> NVAYPLGEGLLSFAESLESQKIHFTTEVITSRIEPANRYVAEKLRITPGQDILYLERLRSIGDEKAMLIENRINIELCPGIVEIDFNQHNLFPTIESLSKRKIRYSESRYAARLIGNERGHFLDISEDAPVLHLEQLVFFSRELPVEFGNVWL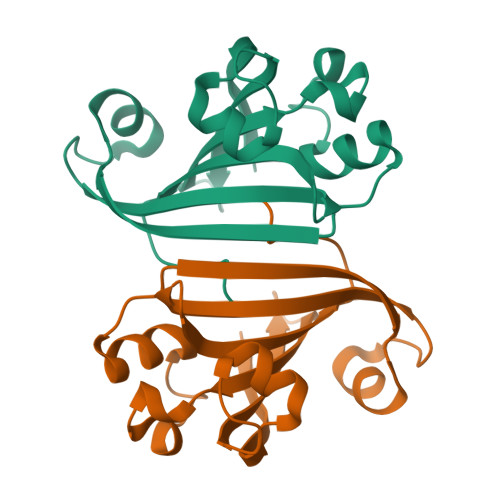KGNKYYLGTVLQRRELS> SNAADPEVCCFITKILCAHGGRMALDALLQEIALSEPQLCEVLQVAGPDRFVVLETGGEAGITRSVVATTRARVCRRKYCQRPCDNLHLCKLNLLGRCNYSQSERNLCKYSHEVLSEENFKVLKNHELSGLNKEELAVLLLQSDPFFMPEICKSYKGEGRQQICNQQPPCSRLHICDHFTRGNCRFPNCLRSHNLMDRKVLAIMREHGLNPDVVQNIQDICNSKHMQKN;> SNAGGIRKTRETERLRRQLLEVFWGQDHKVDFILQREPYCRDINQLSEALLSLNF

ZAP is an antiviral protein that binds to and depletes viral RNA, which is often distinguished from vertebrate host RNA by its elevated CpG content. Of the multiple ZAP cofactors that have been reported, tripartite motif protein 25 (TRIM25) and the KH-like and NYN domain-containing protein (KHNYN) appear especially important for antiviral activity. The ZAP N-terminal RNA binding domain constitutes a minimal core that is essential for antiviral complex activity, and we present a crystal structure of this domain that reveals contacts with the functionally required KHNYN C-terminal domain. We show that KHNYN is an active nuclease that acts in a partly redundant manner with its homolog N4BP1.

We expressed and purified recombinant forms of ZAP-X and the KHNYN CTD and used size-exclusion chromatography (SEC) to test whether the CTD interacts with ZAP-X. Mixing CTD and ZAP-X resulted in a shift in the SEC elution profile relative to either protein alone, indicating a species of higher molecular mass than either CTD or ZAP-X. To determine the molecular details of this interaction, we solved a 2.30-Å crystal structure of ZAP-X bound to KHNYNCTD. Moreover, ZAP-X interacts with a CTD surface opposite the linkage to the NYN domain. Additionally, a hydrophobic patch on KHNYNCTD, including Phe696 and Phe719, binds in a hydrophobic groove on ZAP-X lined by residues Val6, Phe9, Ile30, and Leu32 (Interface 2). Phe655 of KHNYNCTD occupies a hydrophobic pocket of ZAP-X, packed against Gly128. The ZAP-X/KHNYNCTD structure revealed a zinc-binding site formed by the two proteins, with the zinc atom coordinated by ZAP-X Glu29 and His17, KHNYNCTD His692, and a water molecule (Interface 3). The presence of zinc in this site was confirmed by zinc anomalous scattering. In our crystal structure, the KHNYNCTD has the traditional three-helix bundle structure of other CUE ubiquitin binding domains but the previous KHNYNCTD structure has helices of different connectivity, spatial arrangement, and length. Three single amino acid substitutions, at Lys12, His17, and Gly128, reduced or eliminated TRIM25-independent antiviral activity. All variants tested were expressed at similar levels. These results suggest that the KHNYN:ZAP interface observed in the crystal structure contributes to the antiviral activity of ZAP and KHNYN but is likely one of several redundant intermolecular interactions.>[2x]SMEGVIESNWNEIVDSFDDMNLSESLLRGIYAYGFEKPSAIQQRAILPCIKGYDVIAQAQSGTGKTATFAISILQQIELDLKATQALVLAPTRELAQQIQKVVMALGDYMGASCHACIGGT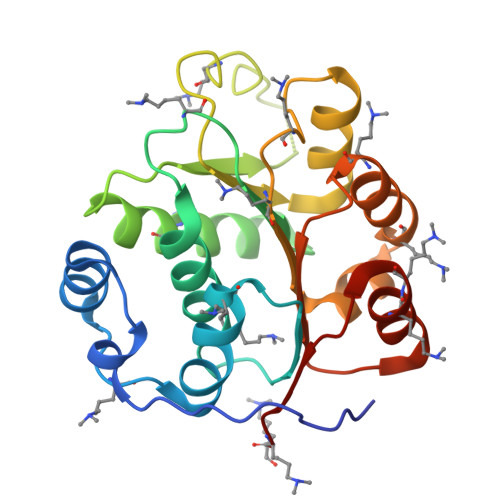NVRAEVQKLQMEAPHIIVGTPGRVFDMLNRRYLSPKYIKMFVLDEADEMLSRGFKDQIYDIFQKLNSNTQVVLLSATMPSDVLEVTKKFMRDPIRILVKK4'-[(2-phenylethyl)carbamoyl][2,2'-bipyridine]-4-carboxylic 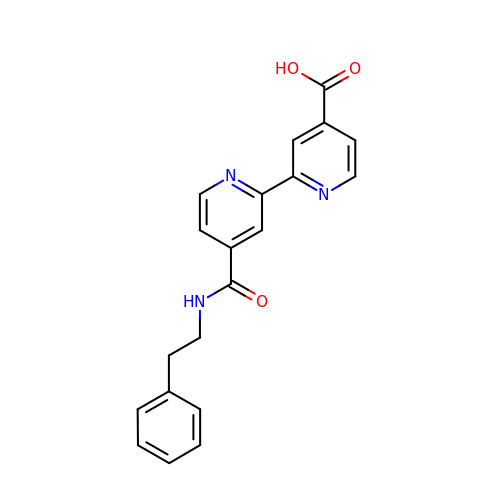acid | C20 H17 N3 O3 | DSGOLESVOJUGOK-UHFFFAOYSA-N> MNKHASQPRAIYYVVALQIWEYFSFYGMRALLILYLTNQLKYNDTHAYELFSAYCSLVYVTPILGGFLADKVLGNRMAVMLGALLMAIGHVVLGASEIHPSFLYLSLAIIVCGYGLFKSNVSCLLGELYEPTDPRRDGGFSLMYAAGNVGSIIAPIACGYAQEEYSWAMGFGLAAVGMIAGLVIFLCGNRHFTHTRGVNKKVLRATNFLLPNWGWLLVLLVATPALITILFW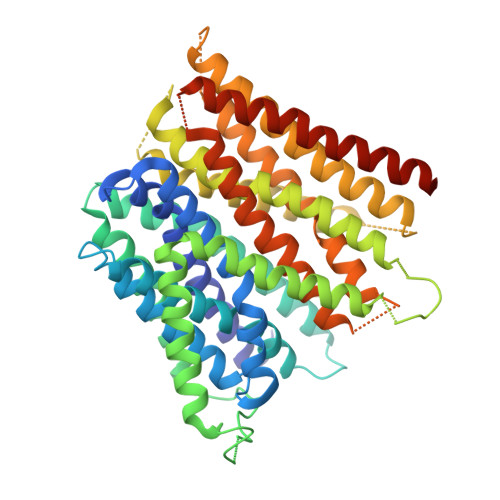KEWSVYALIVATIIGLGVLAKIYRKAENQKQRKELGLIVTLTFFSMLFWAFAQQGGSSISLYIDRFVNRDMFGYTVPTAMFQSINAFAVMLCGVFLAWVVKESVAGNRTVRIWGKFALGLGLMSAGFCILTLSARWSAMYGHSSLPLMVLGLAVMGFAELFIDPVAMSQITRIEIPGVTGVLTGIYMLLSGAIANYLAGVIADQTSQASFDASGAINYSINAYIEVFDQITWGALACVGVVLMIWLYQALKFRNRALALES The most abundant flagellar building block is the flagellin protein that assembles in a helical pattern of more than 20,000 copies to form the extracellular filament. Successful assembly of the flagellar filament relies on the FliS protein that prevents cytoplasmic aggregation of flagellin10 and guides flagellin to the cytoplasmic side of the fT3SS. At the fT3SS, the flagellin/FliS complex interacts with the cytoplasmic domain of the fT3SS transmembrane protein FlhA (FlhA-C). Therefore, FliS acts as targeting factor directing its flagellin client to the export gate of the fT3SS for subsequent secretion.

To obtain the complete structure, the flagellin/FliS complex from B. subtilis was co-expressed in E. coli BL21(DE3) and co-purified by nickel-ion affinity chromatography (IMAC) followed by size exclusion chromatography (SEC). Crystals of the flagellin/FliS complex were obtained in two spacegroups, the primitive monoclinic space group P21 at 1.5 Å resolution and the primitive orthorhombic spacegroup P22121 at 2.1 Å resolution. The flagellin/FliS heterodimer shows overall dimensions of 95 Å, 40 Å and 40 Å and could be built to completeness except for the first 45 highly disordered residues at the N-terminus of flagellin (dashed line). The crystal structure suggests that the flagellin/FliS complex forms a rather compact particle detectable also in solution by small angle X-ray scattering (SAXS). The two proteins interact by an extensive network of hydrophobic and electrostatic interactions with an interface area of 2600 Å2 which can be divided into contact areas 1, 2 and 3. Contact area 1 involves the C-terminus of flagellin (D0-C) wrapped around the surface of FliS in an extended horseshoe like conformation with a mainly hydrophobic interaction area of 1600 Å (Contact area 1). Contact area 1 is highly similar to that in an earlier structure of FliS bound to the C-terminus of flagellin21 with a Cα r.m.s.d of 2.2 Å over 140 amino acid residues. Contact area 2 aligns FliS to the D1 core domain of flagellin, a region that was not present in previous crystal structures. Interactions within this interface are of more electrostatic nature (Contact area 2). Notably, residues 46 to 57 are kinked by 45° in the orthorhombic structure, while the helix is straight in the crystal structure derived from monoclinic crystals. Apart from this difference, both structure superimpose well with a r.m.s.d of 1.5 over 329 Cα-atoms.

> MGHHHHHHRINHNIAALNTLNRLSSNNSASQKNMEKLSSGLRINRAGDDAAGLAISEKMRGQIRGLEMASKNSQDGISLIQTAEGALTETHAILQRVRELVVQAGNTGTQDKATDLQSIQDEISALTDEIDGISNRTEFNGKKLLDGTYKVDTATPANQKNLVFQIGANATQQISVNIEDMGADALGIKEADGSIAALHSVNDLDVTKFADNAADTADIGFDAQLKVVDEAINQVSSQRAKLGAVQNRLEHTINNLSASGENLTAAESRIRDVDMAKEMSEFTKNNILSQASQAMLAQANQQPQNVLQLLR;> MAIQNPYTAYQQNSVNTATPGELTLMLYNGCLKFIRLAAQAIENDDMERKNENLIKAQNIIQELNFTLNRNIELSASMGAMYDYMYRRLVQANIKNDTGMLAEVEGYVTDFRDAWKQAIQSERKDRHGSGGIA> ANIVGGIEYSINNASLCSVGFSVTRGATKGFVTAGHC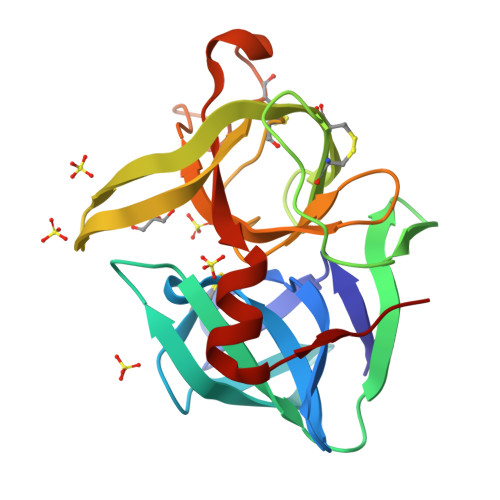GTVNATARIGGAVVGTFAARVFPGNDRAWVSLTSAQTLLPRVANGSSFVTVRGSTEAAVGAAVCRSGRTTGYQCGTITAKNVTANYAEGAVRGLAQGNACMGRGDSGGSWITSAGQAQGVMSGGNVQSNGNNCGIPASQRSSLFERLQPILSQYGLSLVTG>[2x]MDKELGKTLRRLRQGKQVSISSLADEHLSKSQISRFERGESEISSSRLLNLLDKLNITIDEFVSTHSKTHTHFFTLLSRVRKYYAE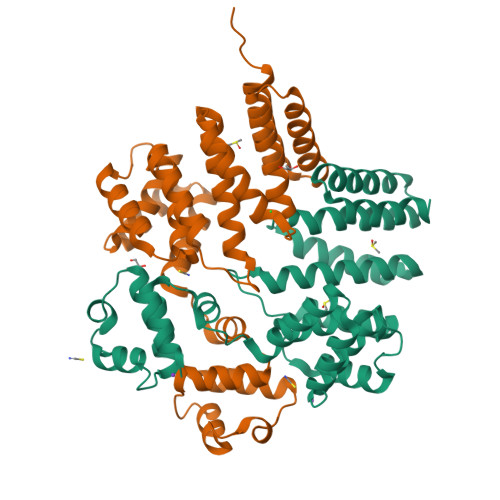KNVAKLLKLLEDYAHKDYESTMIKAILSSIEPTVEPSEEEVTRLTDYLFSVEQWGYYEIILLGNCSRFINYNTLFLLTKEMVTSFAYSEQNKTNKTLVTQLSINCLIISIDYSYFDHSHYLIEKIEFLLRDELNFYEKTVFLYVHGYYKLKQGQVSGKDDMRQALQIFKYLGEDALYYSYKEHYRKEVLGDEED> GSHMGQSLRTLQGHQSAVTSLQFNDNIVVSGSDDSTVKVWDIKTGQSLRTLQGHQSAVTSLQFNDNIVVSGSDDSTVKVWDIKTGQSLRTLQGHQSAVTSLQFNDNIVVSGSDDSTVKVWDIKTGQSLRTLQGHQSAVTSLQFNDNIVVSGSDDSTVKVWDIKTGQSLRTLQGHQSAVTSLQFNDNIVVSGSDDSTVKVWDIKTGQSLRTLQGHQSAVTSLQFNDNIVVSGSDDSTVKVWDIKTGQSLRTLQGHQSAVTSLQFNDNIVVSGSDDSTVKVWDIKTGQSLRTLQGHQSAVTSLQFNDNI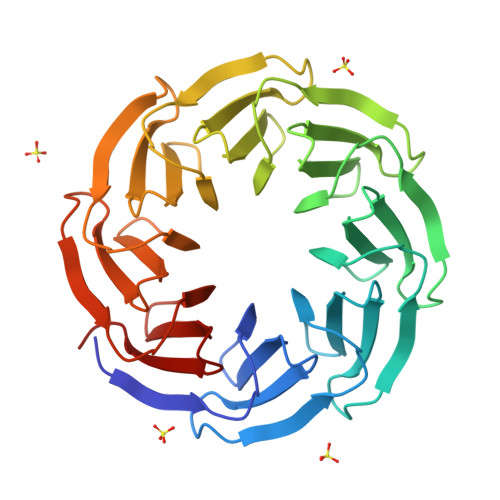VVSGSDDSTVKVWDIKGS>MSDNDELQQIAHLRREYTKGGLRRRDLPADPLTLFERWLSQACEAKLADPTAMVVATVDEHGQPYQRIVLLIHYDEKGMVFYTNLGSRKAHQIENNPRVSLLFPWHTLERQVMVIGKAERLSTLEVMKFFHSLPRDSQIGAWVSKQSSRISARGILESKFLELKQKFQQGEVPLPSFWGGFRVSLEQIEFWQGGEHRLADRFLYQRENDAWKIDRLAP[2x]

In Escherichia coli, PLP formation is catalyzed by pyridoxine 5’-phosphate oxidase (PNPO), a homodimeric FMN-dependent enzyme that is responsible for the last step of PLP biosynthesis and is also involved in the PLP salvage pathway. By using FMN as cofactor, PNPO catalyzes the oxidation of both pyridoxine 5’-phosphate (PNP) and pyridoxamine 5’-phosphate to PLP, reducing molecular oxygen to hydrogen peroxide. We have recently demonstrated that ePNPO undergoes an allosteric feedback inhibition by PLP, through a mechanism in which binding of substrate at the active site and binding of PLP at an allosteric site negatively affect each other to a large extent. We recently showed that an ePNPO quadruple variant (K72I/Y129F/R133L/H199A; ePNPOqm), which has a drastically reduced capability to bind PNP (and therefore PLP) at the active site, is still able to bind PLP at the allosteric site.

The final model of the PLP-bound ePNPOqm (PLP-ePNPOqm) was refined to 2.42 Å resolution; the asymmetric unit contains a 353-residue dimer (residues/chain: 17/A–126/A; 176/A–218/A; 14/B–166/B; 170/B–218/B), one FMN molecule per subunit, one sulphate ion in subunit A, one PLP molecule with 0.81 occupancy in subunit B, and 45 water molecules. In contrast to the symmetrical ePNPOqm structure, the PLP-ePNPOqm is the first ever characterized structure of the enzyme crystallized in a P61 space group, in which the dimer is asymmetric. In the PLP-ePNPOqm model, the subunit A backbone displays a major break of 49 residues (comprising residues 127–175), corresponding to the ePNPO smaller domain comprising the H3, H4, and H5 helices, whereas only a minor break of three residues is present in subunit B (residues 167–169), which could not be modelled because of the lack of information from the FO – FC map. The disorder of these elements in subunit A seems to occur as a consequence of PLP binding in a surface cleft, placed in part at the interface between subunits A and B, mainly circumscribed by three arginine residues (Arg23, Arg24, Arg215) belonging to subunit B and acting as an electrostatic “Arg cage” for PLP. In addition, a small network of hydrogen bonds takes place between Arg23 and the PLP phosphate group by means of a bridging water molecule, HOH419, whose role is apparently to contribute to stabilizing PLP lodging in the cavity; this effect is enhanced by the pyridine ring, able to coordinate Arg24 and Arg215 via the deprotonated nitrogen atom. The superimposition of PLP-ePNPOqm and ePNPOqm revealed important differences between the two structures, highlighting the structural change induced by PLP binding to the allosteric site. Indeed, PLP binding causes the dismantling of a specific pattern of hydrogen bonds and electrostatic interactions anchoring H5 of subunit A to a short neighboring protein segment made of residues 192 to 200 of subunit B (“H-unc”).>[2x]GSAKDPMKGRDVVLGLLMQKELSGYDIKIVFEDVFTHFFDGSFGMIYPTLRQLENEGKIKKEVVMQEGKPNKKMYFITDEGREEFYQYMQTPVEKDVLRSDFLMRMYFGNYS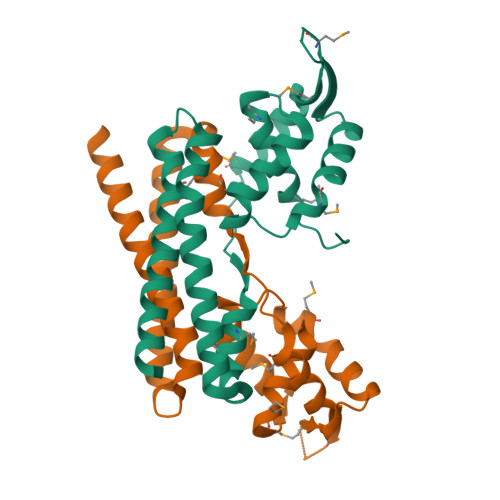DDVTIKKWIKDEIERKEAYIADLRLKYEKWRVGITFVEEISLDVGIASYSAQVETLKKKLEELEAKENNKTEE4-{2-[(1R)-2-{(carboxymethyl)[(thiophen-2-yl)methyl]amino}-2-oxo-1-{[(2-oxo-1,2-dihydroquinolin-6-yl)sulfonyl]amino}ethyl]phenoxy}butanoic acid | C28 H27 N3 O9 S2 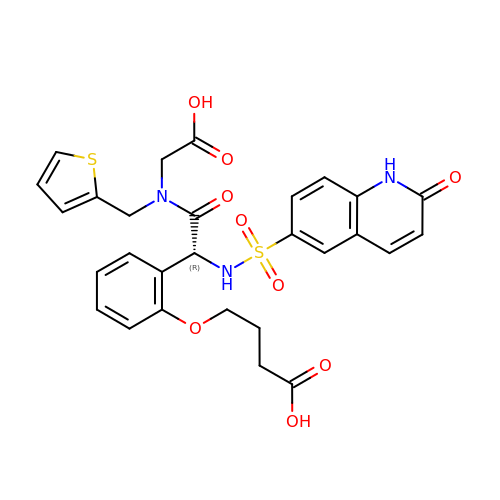| XMWFXIHFGQHVEA-HHHXNRCGSA-N>YGFNKCTQYEFDIHHVLCIRKKITNLTEAISDIPRYTTHLNLTHNEIQVLPPWSFTNLSALVDLRLEWNSIWKIDEGAFRGLENLTLLNLVENKIQSVNNSFEGLSSLKTLLLSHNQITHIHKDAFTPLIKLKYLSLSRNNISDFSGILEAVQHLPCLERLDLTNNSIMYLDHSPRSLVSLTHLSFEGNKLRELNFSALSLPNLTNLSASRNGNKVIQNVYLKTLPQLKSLNLSGTVIKLENLSAKHLQNLRAMDLSNWELRHGHLDMKTVCHLLGNLPKLETLVFQKNVTNAEGIKQLAKCTRLLFLDLGQNSDLIYLNDSEFNALPSLQKLNLNKCQLSFINNRTWSSLQNLTSLDLSHNKFKSFPDFAFSPLKHLEFLSLSRNPITELNNLAFSGLFALKELNLAACWIVTIDRYSFTQFPNLEVLDLGDNNIRTLNHGTFRPLKKLQSLILSHNCLKILEPNSFSGLTNLRSLDLMYNSLSYFHEHLFSGLEKLLILKLGFNKITYETTRTLQYPPFIKLKSLKQLNLEGQRHGIQVVPSNFFQGLGSLQE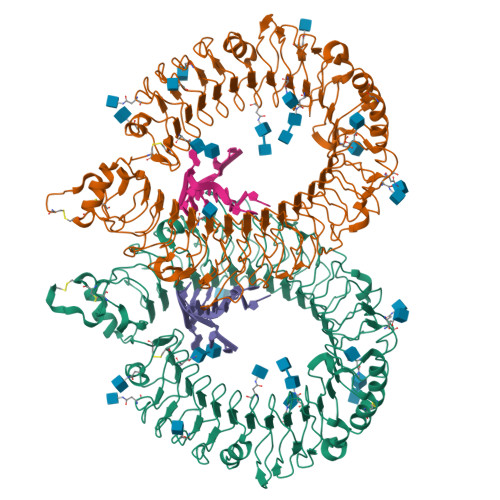LLLGKNPSVFLDHHQFDPLINLTKLDISGTKDGDRSLYLNASLFQNLKRLKILRLENNNLESLVPDMFSSLQSLQVFSLRFNNLKVINQSHLKNLKSLMFFDVYGNKLQCTCDNLWFKNWSMNTEEVHIPFLRSYPCQQPGSQSLLIDFDDAMC[2x]> GSQIPASEQETLVRPKPLLLKLLKSVGAQKDTYTMKEVLFYLGQYIMTKRLYDEKQQHI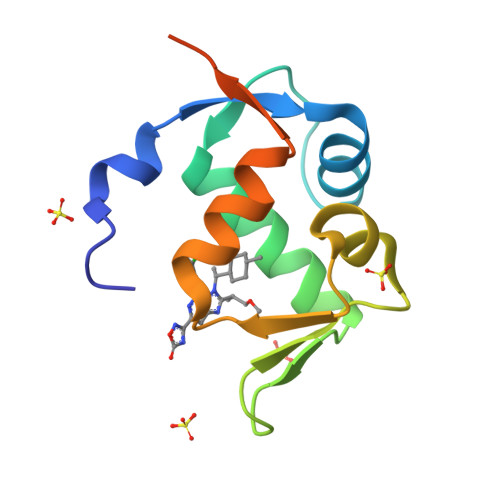VYCSNDLLGDLFGVPSFSVKEHRKIYTMIYRNLVVVNQQESSDSGTSVSEN> RTHRL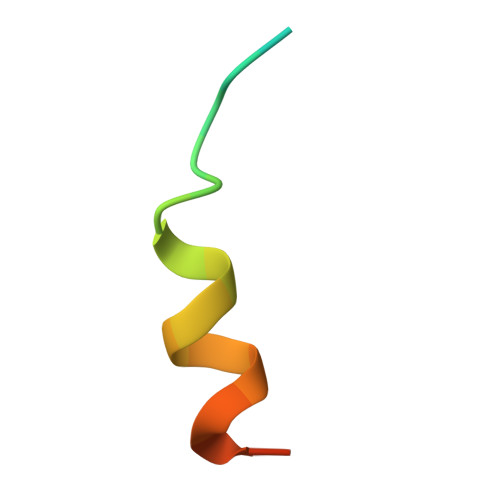ITLADHICQIITQDFARN6-(4-methylpiperazin-1-yl)-N-(5-methyl-1H-pyrazol-3-yl)-2-[(E)-2-phenylethenyl]pyrimidin-4-amine 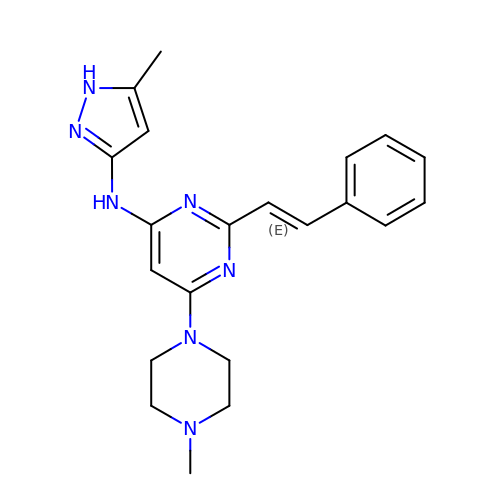| C21 H25 N7 | BLQYVHBZHAISJM-CMDGGOBGSA-N>DPSKDSKAQVSAAEAGITGTWYNQLGSTFIVT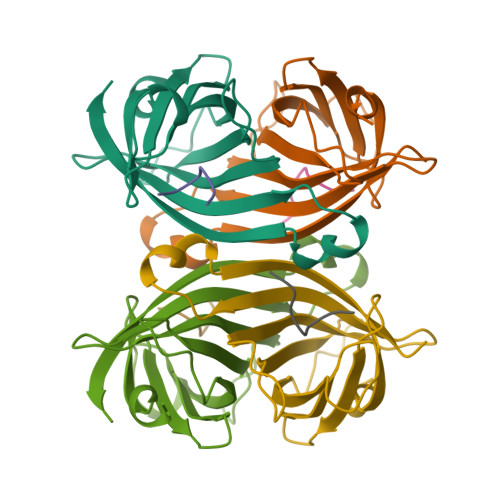AGADGALTGTYESAVGNAESRYVLTGRYDSAPATDGSGTALGWTVAWKNNYRNAHSATTWSGQYVGGAEARINTQWLLTSGTTEANAWKSTLVGHDTFTKVKP[2x];>[2x]FSHPQNT4-deoxy-L-threo-hex-5-ulosuronic acid 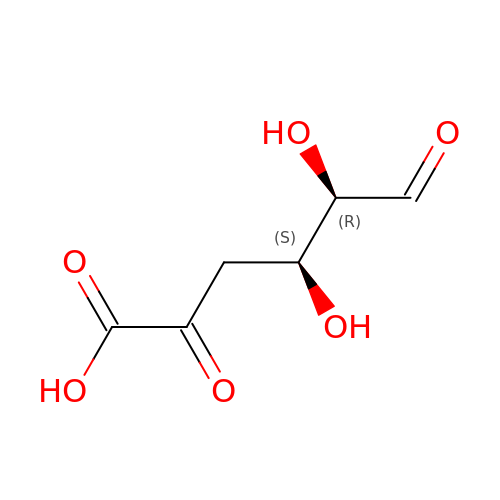| C6 H8 O6 | IMUGYKFHMJLTOU-UCORVYFPSA-N> CG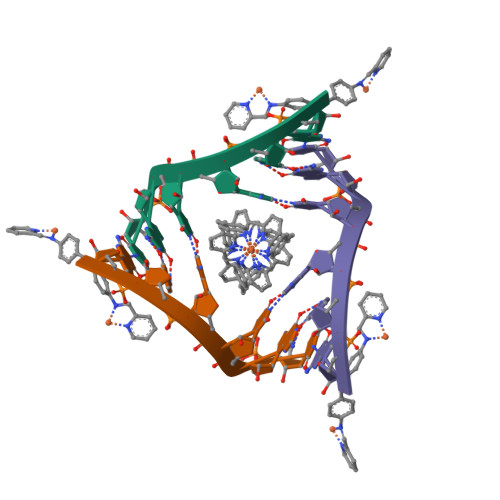UACG> SNAGKKNE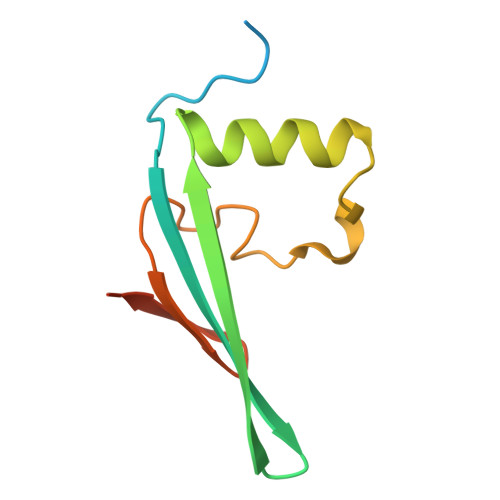DSGEPVYISRYSSLVPIEKVGFTLKNEINSRIITIKLKFNGNDIFGGLHELCDKNLINIDKVPGWLAGENGSFSGTIMNGDFQREQVAKGGLL>MTGARASAAEQRRAGRSGQARAAERAAGMSGAGRALAALLLAASVLSAALLAPGGSSGRDAQAAPPRDLDKKRHAELKMDQALLLIHNELLWTNLTVYWKSECCYHCLFQVLVNVPQSPKAGKPSAAAASVSTQHGSILQLNDTLEEKEVCRLEYRFGEFGNYSLLVKNIHNGVSEIACDLAVNEDPVDSNLPVSIAFLIGLAVIIVISFLRLLLSLDDFNNWISKAISSRETDRLINSELGSPSRTDPLDGDVQPATWRLSALPPRLRSVDTFRGIALILMVFVNYGGGKYWYFKHASWNGLTVADLVFPWFVFIMGSSIFLSMTSILQRGCSKFRLLGKIAWRSFLLICIGIIIVNPNYCLGPLSWDKVRIPGVLQRLGVTYFVVAVLELLFAKPVPEHCASERSCLSLRDITSSWPQWLLILVLEGLWLGLTFLLPVPGCPTGYLGPGGIGDFGKYPNCTGGAAGYIDRLLLGDDHLYQHPSSAVLYHTEVAYDPEGILGTINSIVMAFLGVQAGKILLYYKARTKDILIRFTAWCCILGLISVALTKVSENEGFIPVNKNLWSLSYVTTLSSFAFFILLVLYPVVDVKGLWTGTPFFYPGMNSILVYVGHEVFENYFPFQWKLKDNQSHKEHLTQNIVATALWVLIAYILYRKKIFWKI[2x]

Before the glycosidases can act, the terminal glucosamine of HS must be acetylated by the integral lysosomal membrane enzyme heparan-α-glucosaminide N-acetyltransferase (HGSNAT). HGSNAT catalyzes a unique transmembrane acetylation reaction where the acetyl group of cytosolic acetyl-CoA is transported across the lysosomal membrane and attached to HS in one reaction. We find that a central pore within each monomer traverses the membrane and controls access of cytosolic acetyl-CoA to the active site at its luminal mouth where glucosamine binds. A histidine-aspartic acid catalytic dyad catalyzes the transfer reaction via a ternary complex mechanism.

Rather, the acetyl-CoA binding site forms a continuous positively charged pore as the binding pocket that allows it to transverse the TMD and position the acetyl group at the active site at the luminal mouth. Acetyl-CoA binding then fully opens the pore and positions the acetyl group at the active site located at the luminal mouth of it in the priming state. This configuration of the substrates binding and the active site is the structural basis for the transmembrane acetylation reaction. The CoA moiety interacts with HGSNAT through an extensive network of polar and hydrophobic interactions: a large number of polar interactions at the cytosolic mouth stabilize the 3’-phosphoadenosine, while R345 and R275 form hydrogen/ionic bonds with the diphosphate; the pantothenate group is accommodated through hydrophobic interactions, while the cysteamine forms a hydrogen bond with M282. The carbonyl of the acetyl group is stabilized by N286, whose mutation is identified in MPS patients. In addition, N286 is positioned 2.7 Å away from the carbonyl oxygen of the acetyl group, which stabilizes the negative charge in the intermediate state. Aside from being an integral part of the reaction cycle, the lack of extra density representing the acetyl group in the [CoA] structure compared to the [Acetyl-CoA] structure helped us to precisely model the position of the Acetyl group. The ligand(s) bound structures as well as the Apotrans structure adopt similar structures with a dilated configuration where Y361 folds back into the interface and interactions are mostly hydrophobic.> GDKDNGLHAGETDGDDEGFEFRRH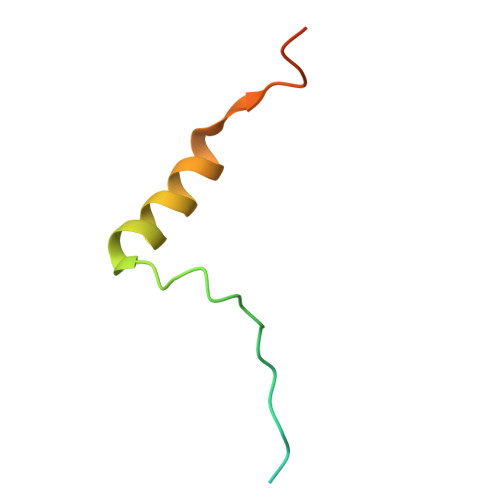SNLGVPTLGERLDSLHEIKSARRMDHFNSSRNSLR> XAPSYSPP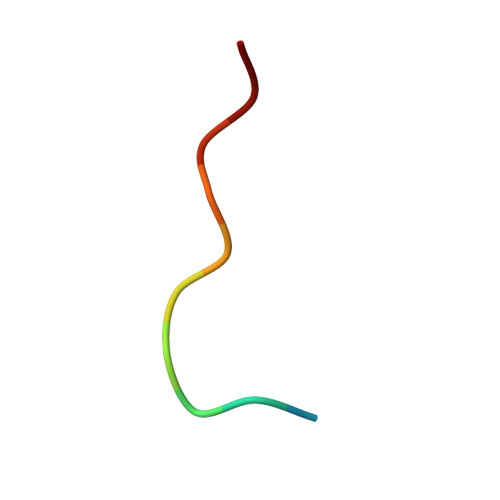PPP> GPMDFLRSLDWTQVIAGQYVSNPRFNISDYFEIVRQPGDGNCFYHSIAE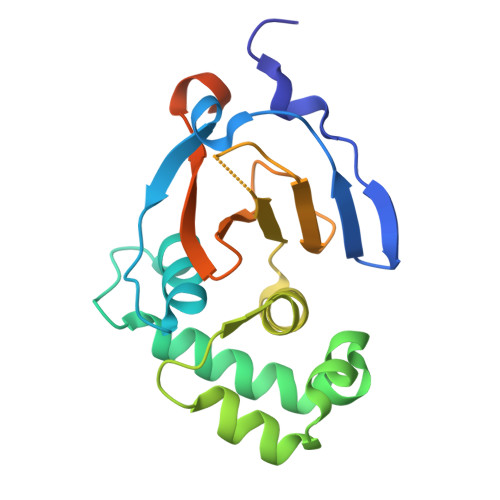LTMPNKTDHSYHYIKRLTESAARKYYQEEPEARLVGLSLEDYLKRMLSDNEWGSTLEASMLAKEMGITIIIWTVAASDEVEAGIKFGDGDVFTAVNLLHSGQTHFDALRILPQFETDTREALSLMDRVIAVDQLTS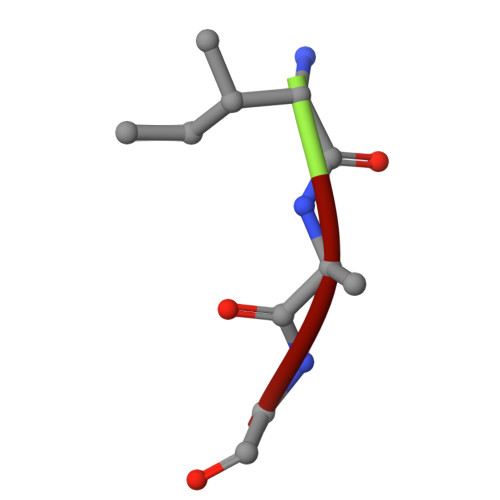> IAG> MHHHHHHQIGWRREGIKYRRNELFLDVLESVNLLMSPQGQVLSAHVSGRVVMKSYLSGMPECKFGMNDKIVIEKQGKGTADETSKSGKQSIAIDDCTFHQCVRLSKFDSERSISFIPPDGEFELMRYRTTKDIILPFRVIPLVREVGRTKLEVKVVIKSNFKPSLLAQKIEVRIPTPLNTSGVQVICMKGKAKYKASENAIVWKIKRMAGMKESQISAEIELLPTNDKKKWARPPISMNFEVPF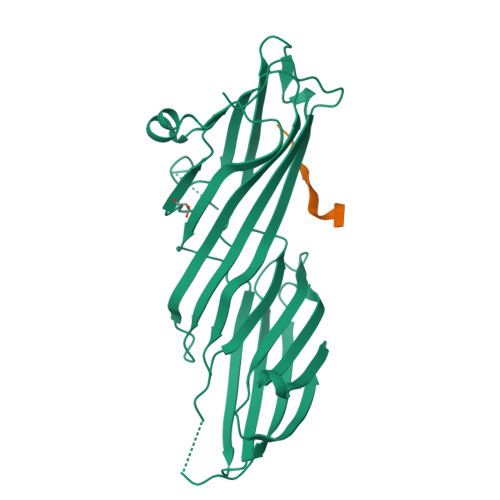APSGLKVRYLKVFEPKLNYSDHDVIKWVRYIGRSGIYETRC;> SDLLAWDPLFG> MRDIVFVSPQLYLSSQEGWKSDSAKSGFIPILKNDLQRFQDSLKHIVDARNSLSETLLNSNDDGSIHNSDQNTGLNKDKEASIADNN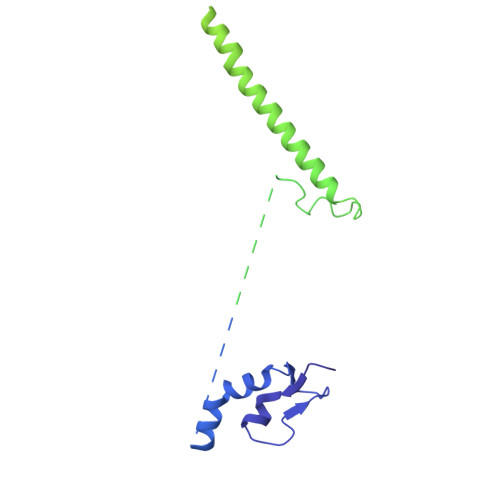SANKCATSSSRYQELKQFLPISLDQQIHTVSLQGVSSSFSRGQIESLLDHCLNLALTETQSNSALKVEAWSSFSSFLDTQDIFIRFSKVDEDEAFVNTLNYCKALFAFIRKLHEDFKIELHLDLNTKEYVEDRTGTIPSVKPEKASEFYSVFKNIEDQTDERNSKKEQLDDSSTQYKVDTNTLSDLPSDALDQLCKDIIEFRTKVVSIEKEKKMKSTYEESRRQRHQMQKVFDQIRKNHSGAKGSANTEEEDTNMEDEDEEDDTEDDLALEKRKEERDLEESNRRYEDMLHQLHSNTEPKIKSIRADIMSAENYEEHLEKNRSLYLKELLHLANDVHYDHHRSFKEQEERRDEEDRAKNGNAKELAPIQLSDGKAISAGKAAAITLPEGTVKSENYNADKNVSESSEHVKIKFDFKKAIDHSVESSSEDEGYRESELPPTKPSERSAAEDRLPFTADELNIRLTNLKESRYVDELVREFLGVYEDELVEYILENIRVNQSKQALLNELRETFDEDGETIADRLWSRKEFRLGT> GSHMSAGIGESRTELLTWLNGLLNLNYKKIEECGTGAAYCQIMDSIYGDLPMNRVKFNAT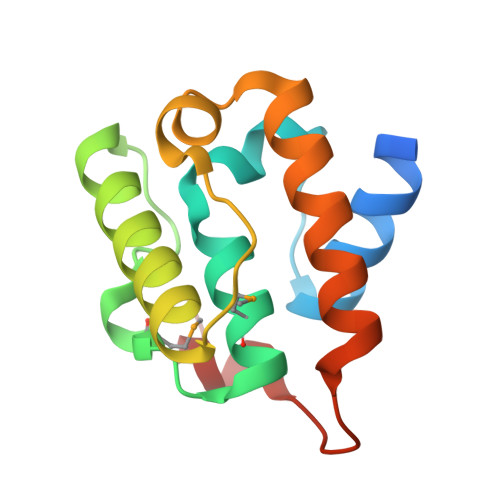AEYEFQTNYKILQSCFSRHGIEKTVYVDKLIRCKFQDNLEFLQWLKKHWIRHKDESVYDPDARRKYR> MALKGNMQVENLEAVEDPQVDLGAQVSAAPRAKRQARQAEDVQG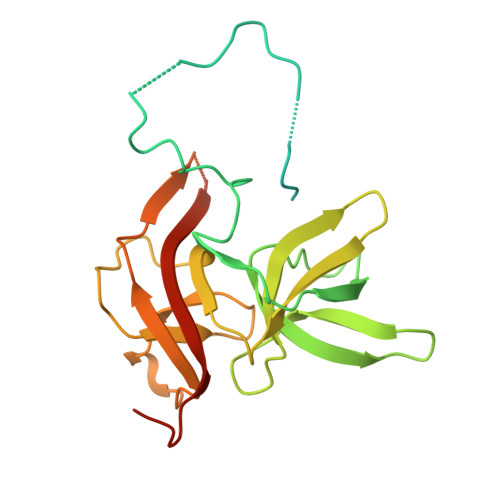EDPYLESISELDDVLLKFKKYSKSMSSIENKVFSSSSGCFKSKNERVDAYSFACSSYTDKIEEYLYDPANSFPYKRGVKLVPKENSIYVEVGADTDMYGICVDVCEFSCTAYVLPITNNFEGYLVTRNPSIKIGEILDINNNGVIIKAGGGPPTAINIYALSDSFTINFAPEDGNQDQNRYPRQEYSINLIKVAIFGNRGLEKTVNPDGG>MVQKESQATLEERESELSSNPAASAGASLEPPAAPAPGEDNPAGAGGAAVAGAAGGARRFLCGVVEGFYGRPWVMEQRKELFRRLQKWELNTYLYAPKDDYKHRMFWREMYSVEEAEQLMTLISAAREYEIEFIYAISPGLDITFSNPKEVSTLKRKLDQVSQFGCRSFALLFDDIDHNMCAADKEVFSSFAHAQVSITNEIYQYLGEPETFLFCPTEYCGTFCYPNVSQSPYLRTVGEKLLPGIEVLWTGPKVVSKEIPVESIEEVSKIIKRAPVIWDNIHANDYDQKRLFLGPYKGRSTELIPRLKGVLTNPNCEFEANYVAIHTLATWYKSNMNGVRKDVVMTDSEDSTVSIQIKLENEGSDEDIETDVLYSPQMALKLALTEWLQEFGVPHQYSSRQVAHSGAKASVVDGTPLVAAPSLNATTVVTTVYQEPIMSQGAALSGEPTTLTKEEEKKQPDEEPMDMVVEKQEETDHKNDNQILSEIVEAKMAEELKPMDTDKESIAESKSPEMSMQEDCISDIAPMQTDEQTNKEQFVPGPNEKPLYTAEPVTLEDLQLLADLFYLPYEHGPKGAQMLREFQWLRANSSVVSVNCKGKDSAKIAEWRSRAAKFEEMCGLVMGMFTRLSNCANRTILYDMYSYVWDIKSIMSMVKSFVQWLGCRSHSSAQFLIGDQEPWAFRGGLAGEFQRLLPIDGANDLFFQPPPLTPTSKVYTIRPYFPKDEASVYKICREMYDDGVGLPFQSQPDLIGDKLVGGLLSLSLDYCFVLEDEDGICGYALGTVDVTPFIKKCKISWIPFMQEKYTKPNGDKELSEAEKIMLSFHEEQEVLPETFLANFPSLIKMDIHKKVTDPSVAKSMMACLLSSLKANGSRGAFCEVRP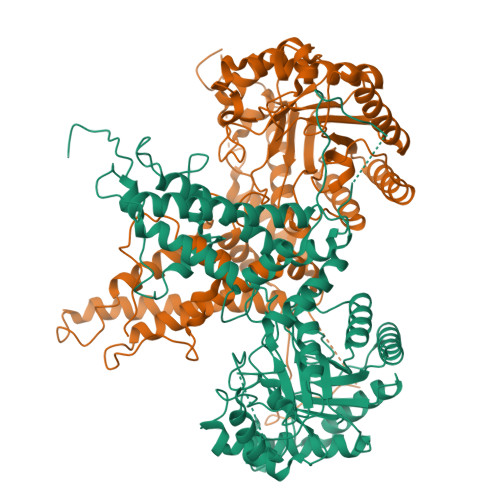DDKRILEFYSKLGCFEIAKMEGFPKDVVILGRSL[2x]>AMALEARLEQASILKKVVDAIKDLVQDCNFDCNDSGIALQAMDNSHVALVSMMLKAEGFSPYRCDRNIALGVNLTSLTKVLRAAQNEDILTLKAEDAPDVLNLVFESSETDRISEYDLKLMDIDQEHLGIPETEYAATITMPSNEFKRITTDLMAMSESVTIEANKDGVKFSCQGDIGNGSVTLRQHTNVEKPNESIEIELSEPVSLTFSLKYLVNFCKASALSNTVKICLSNEVPLLVEYSLGGSSYLRFYLAPKIGDDE[6x];>KHQSTLNFKHRVTKP[4x]

DNA polymerase δ (Pol δ) is a key enzyme for the maintenance of genome integrity in eukaryotic cells, acting in concert with the sliding clamp processivity factor PCNA (proliferating cell nuclear antigen). Three of the four subunits of human Pol δ interact directly with the PCNA homotrimer via a short, conserved protein sequence known as a PCNA interacting protein (PIP) motif.

Here, we describe the identification of a PIP motif located towards the N terminus of the PolD4 subunit of Pol δ (equivalent to human p12) from the thermophilic filamentous fungus Chaetomium thermophilum and present the X‐ray crystal structure of the corresponding peptide bound to PCNA at 2.45 Å. Like human p12, the fungal PolD4 PIP motif displays non‐canonical binding to PCNA. However, the structures of the human p12 and fungal PolD4 PIP motif peptides are quite distinct, with the fungal PolD4 PIP motif lacking the 310 helical segment that characterises most previously identified PIP motifs. Instead, the fungal PolD4 PIP motif binds PCNA via conserved glutamine that inserts into the Q‐pocket on the surface of PCNA and with conserved leucine and phenylalanine sidechains forming a compact 2‐fork plug that inserts into the hydrophobic pocket on PCNA. Despite the unusual binding mode of the fungal PolD4, isothermal calorimetry (ITC) measurements show that its affinity for PCNA is similar to that of its human orthologue. These observations add to a growing body of information on how diverse proteins interact with PCNA and highlight how binding modes can vary significantly between orthologous PCNA partner proteins.> MKNWQRIVEAKLEQQKHKVAEISLENGTVNYSKKIKHNRNLKALTGDEEIVRAFLIDRLVNELDYKPEYLETEKEYTIKGGHSKINPRVDVLVKDDKGNPFFFIEVKAPNKFEEDKDEIEGQLFALAQAEERDFKTKVKYLVYYTVELIDDEIVDRAIIIDFEKYPTYTDWSNGGFISTGTELTAGYGEPKKQPLIKGHEKYDLRVRIDREEIEGLGRNLHNVLWGGGGTNDSEIFYSLVNIILAKIQDEYEKEDGQEYDFQVYQYGDNVESPQKLFDRINALYKRALREQLNVTDEQKIAEDNVINRNKFPLNKLVYTVQALESLSFLEGRNSLDGKDILGDFFESIIRDGFKQTKGQFFTPTPIVKFILYALQLDKLAIDRLNNDRELPLIIDPSAGSGTFLIEAMKLITKEVKYKQNHKVKSSRQITKRFEELFMPDHNENKWAREYLYGCEINFDLGTASKVNMILHGDGSANIFVQDGLLPFRFYVKETSPNYLETASPDALYGDKEVNGKFDVVVSNPPFSVDLDTQTQREVRNAFLFGDKKNSENLFIERYYQLLKEGGRLGVVLPESVFDTTENKYIRLFIFKYFKVKAVVSLPQVTFEPFTSTKTSLLFAQKKTKEEVEQWNELWDKYGKEWSLLKTRINDYFSYFVKGRPLNKKWAPDVVKDIQEGNEDNIRKNIFRFLKDHIKEEDKNLEIKDLLIKYAEEISSISKHEKETDVFGFYNAWWVFGEVAKELDYPIFMAEAENVGYKRTKKGEKPMPNDLYDLEYAPSTLDCEKVLSSFDIEINALEASKTKLSVEKGLLEEKLKDKEDKENEKIQKRLNKISELLETIENQLDSIRSKKLEVEGILEKYYENNKLKEEYSERDDEELINHFKHGVLYQY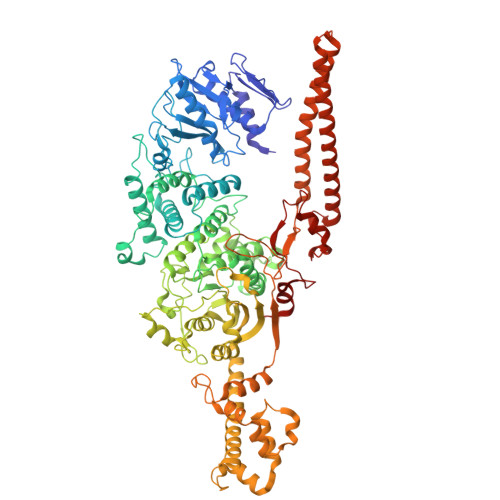RSEDILLRNKTVHKILDEIRQGVIWD> KAT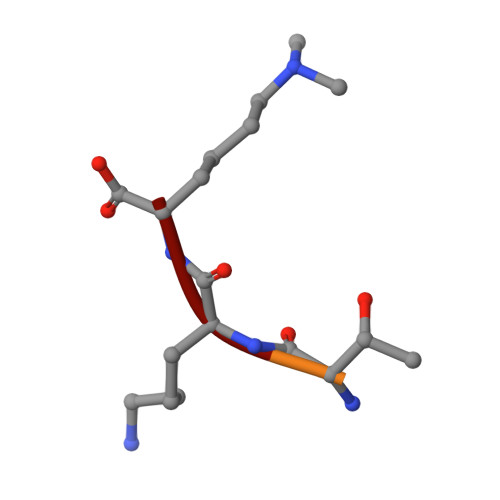KK> HMASMTGGQQMGRMSHMRPAFGAAWN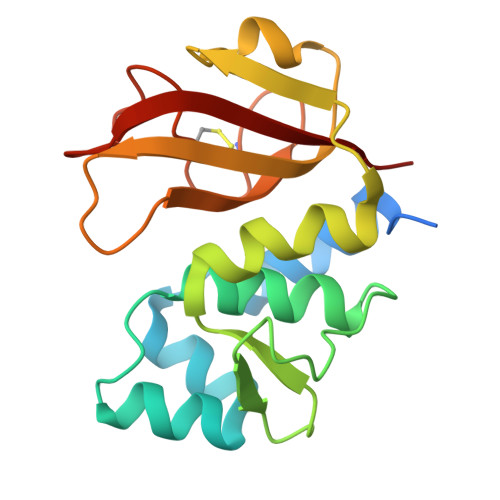RFKEVNVNVEQVGKLLGGKVQHNIDAGIFKNACPIRMSYVLNYCGIPVPSNSKYATVTGSDKKRYMFRVKDMIAFLPTVLGKADISVSSPTPAQFAGKQGIIIFTGHGWLDATGHVTLWNGNICSDDCHFLGSPGNGSFIPTNATFWSLK(2S,3R,4S)-2-[(2S,3R)-1,3-bis(oxidanyl)-1-oxidanylidene-butan-2-yl]-4-[1-(4,5-dihydro-1,3-thiazol-2-yl)azetidin-3-yl]sulfanyl-3-methyl-3,4-dihydro-2H-pyrrole-5-carboxylic 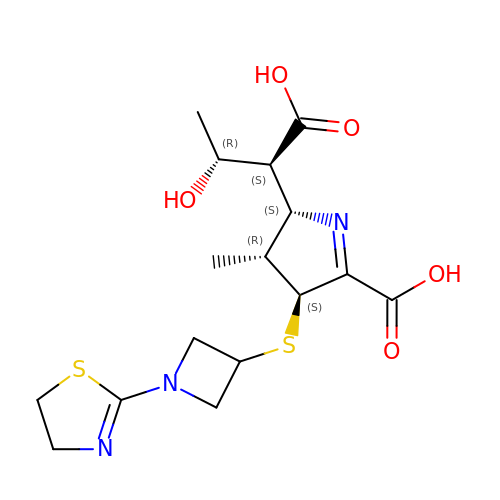acid | C16 H23 N3 O5 S2 | FOPUWSKGBIXNGQ-NSOMGTDFSA-N>[2x]MGSSHHHHHHSSGENLYFQGHMSSTFEPATDSPLPVPGVQYFLQHVQSGKYVHPHGGSDMPGNDTALVLHHGFDEKRDALRWVFVNDAENKHQLKHYSSGKFVHPKGGKVGKEATLVVHSSPGRPETMIEMVQEDGRTYLRHTDSDYYVHPHGGSPNPGDNTRLVYYSGYRPSLAFLAIPAETLFVDRIEIHQAQALESINTITSLSDEHRNDTDQPVQTSISVALEESLQDSAQLSFERCFGLKVGSEFEVGLPLVGKTKVSVQFSGSWKSSTIKGEVRTSAVKVQINEHVTIPPGKCVQIRIDTRRCTKTAPATMYLRTASGIEVQRETTVTSTYHYDQEVHVVPVTN

TrefLec was searched for original domain combinations, which led to single out SaroL-1 in the choanoflagellate Salpingoeca rosetta, that contains both β-trefoil and aerolysin-like pore-forming domains. Recombinant SaroL-1 is shown to bind galactose and derivatives, with a stronger affinity for cancer-related α-galactosylated epitopes such as the glycosphingolipid Gb3, when embedded in giant unilamellar vesicles or cell membranes. SaroL-1 is composed of two domains, a β-trefoil domain at the N-terminal region shown in blue and an elongated domain (green) consisting of seven β-strands forming a twisted β-sheet. The lectin-binding step is necessary for the pore-formation since the pre-incubation with a high affinity galactose derivative diminishes or abolishes hemolysis, GUVs penetration, and cytotoxicity.

Attempts to solve the crystal structures by molecular replacement were unsuccessful. Thus the selenium-methionine variant of SaroL-1 was expressed, purified, and crystallized for experimental determination of the phases. The monosaccharides N-acetylgalactosamine (GalNAc) and α-methyl galactoside (GalαOMe) displayed a similar millimolar affinity with a Kd of 2.2 and 2.8 mM, respectively. Clear electron density for three GalNAc monosaccharides is observed in the lectin domain, corresponding to the three sites α, β and γ, classically observed in the β-trefoil structure. The axial O4 of αGalNAc establishes hydrogen bonds with the side chain of conserved His and Arg residues in all sites. Moreover, each GalNAc is stabilized in the binding pocket by a C-π-stacking interaction between its hydrophobic face and the aromatic ring of His (site α and β) or Tyr (site γ).5-cyano-2'-{4-[2-(3-methyl-1H-indol-1-yl)ethyl]piperazin-1-yl}-N-[3-(pyrrolidin-1-yl)propyl]biphenyl-3-carboxamide | C36 H42 N6 O | 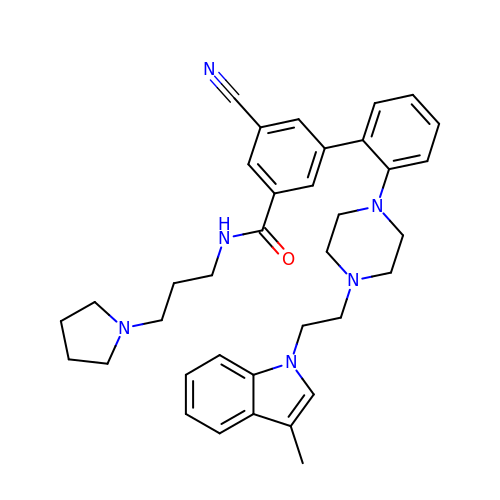PNYRDVBFYVDJJI-UHFFFAOYSA-N> SHMKSFFDKKRSERISNGGFRPAAPNLAGAVEFSDVKTLLKEWITTISDPMEEDILQVVRYCTDLIEEKDLEKLDLVIKYMKRLMQQSVESVWNMAFD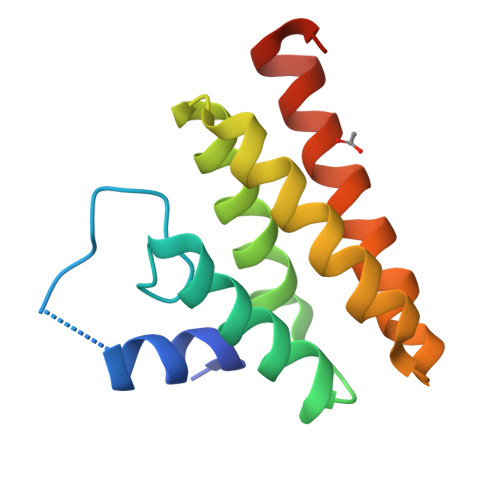FILDNVQVVLQQTYGSTLKVT8-amino-7-chloro-1-methyl-6-(methylideneamino)-2-oxo-1,2-dihydropyrrolo[4,3,2-de]quinoline-4-carboxamide | C13 H10 Cl N5 O2 | 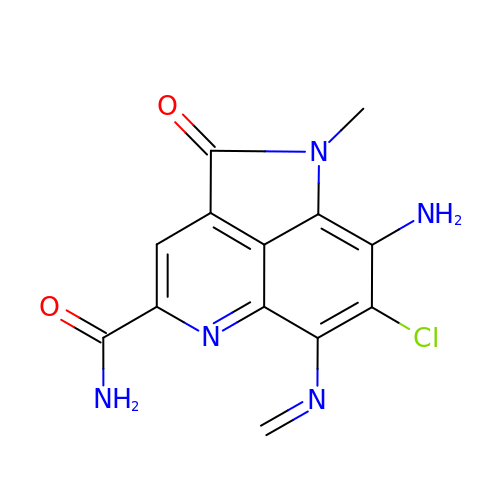IRLASAQBVTZKMT-UHFFFAOYSA-N(E)-N-{2-hydroxy-3-methyl-6-[(phosphonooxy)methyl]benzylidene}-L-aspartic 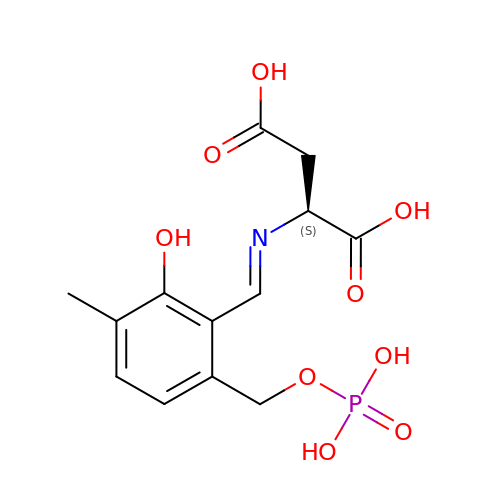acid | C13 H16 N O9 P | CMDDKMGWJXISQE-ZFGNZVLRSA-N> MSERIVPSGDVELWSDDFGDPADPALLLVMGGNLSALGWPDEFARRLADGGLHVIRYDHRDTGRSTTRDFAAHPYGFGELAADAVAVLDGWGVDRAHVVGLSMGATITQVIALDHHDRLSSLTMLLGGGLDID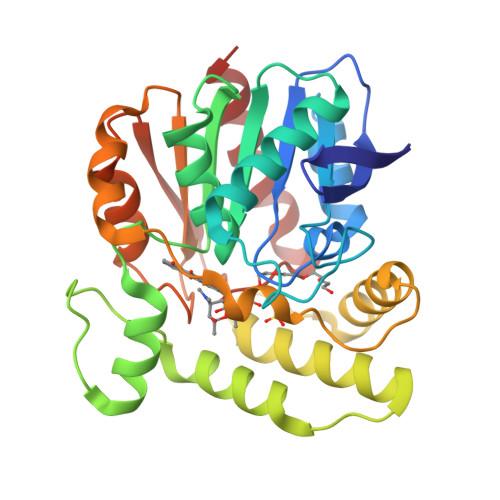FDANIERVMRGEPTLDGLPGPQQPFLDALALMNQPAEGRAAEVAKRVSKWRILSGTGVPFDDAEYARWEERAIDHAGGVLAEPYAHYSLTLPPPSRAAELREVTVPTLVIQAEHDPIAPAPHGKHLAGLIPTARLAEIPGMGHALPSSVHGPLAEVILAHTRSAA Here we report a structural and functional analysis for an epimerase, KasQ, that primes KSM biosynthesis rather than the previously proposed KasF/H, which instead acts as an acetyltransferase, inactivating KSM. Our biochemical and biophysical analysis determined that KasQ converts UDP-GlcNAc to UDP-ManNAc as the initial step in the biosynthetic pathway. To better understand the catalytic mechanism of KasQ, we solved crystal structures of KasQ for the wild type (WT) and its complexes with UDP or UDP-Glc in resolutions of 2.44 Å, 2.58 Å, and 2.09 Å, respectively. In brief, each monomer consists of two domains (N-terminal and C-terminal domains), in which each subdomain is made of a typical sandwich (αβα) architecture of a Rossmann fold.

In consistence with homodimers in solution, an asymmetric unit contains two monomers colored in rainbow (N-terminal blue, C-terminal red) and gray. Superimposition of these two monomers with an RMSD of 0.86 Å for 317 Cα atoms indicated no significant conformational differences. Two fragments marked in dashed lines (residues 40–45 in the N-terminal domain and residues 184–190 in the C-terminal domain) are missing from the model due to lack of electron density, likely a consequence of structural disorder/flexibility in loop regions. The N-terminal domain is constituted by residues 1–170 that fold into a central seven-strand β-sheet (β1–β7) sandwiched by α-helices (α1–α7) on each side along with a stand-alone α16 helix (residues 357–370). The C-terminal domain is formed by residues 201–359 composed of a central six-strand β-sheet (β8–β13) sandwiched α-helices (α9–α16) on each side. The N-terminal and C-terminal domains are connected by two helices, α7–α8 (residues 173–199). The cleft between these two domains provides the substrate binding pocket. A sodium ion was observed in coordination with the carbonyl backbone of N-terminal residues Leu25, Asp26, Asp28, and Phe31.

>[2x]MALRVGIVYGTRPEAIKLAPLVLALDADPGFEPVIITTGQHRDMLDEINELFGLRPRHNLDIMRPGQRLSAMASRIVGELGDPLLDELVDVAVVQGDTSTAFAAAYAAACERIPVAHLEAGLRTGDRFEPFPEEINRRLITQLADLHFAPTADAAGNLLAEGVRSDDVYVTGNTVIDAMHLVLDRPGDSANRELDAFTEGRQTVLLTMHRRESWGIPMGRVAAAVAELCRSRPTLRFVIPLHPNPEVRRVFRSHLSSLTQVLLCEPLRYSEFIRLMHRAVLVLTDSGGVQEEAPTLGKPVLVLRDRTERPEGIAAGCARLVGTDPALIVKEVGRLLDDPEAYEAMRRPGIVCYGEGDAAARCLEALRERWLSSPDASAGLRTYR>GFKQDIATLRGDLRTYAQDIFLAFLNKFPDEKRNFKNYVGKSDQELKSMAKFGDHTEKVFNLMMEVADRATDCVPLASDASTLVQMKQHSGLTTGNFEKLFVALVEYMRASGQSFDSQSWDRFGKNLVSA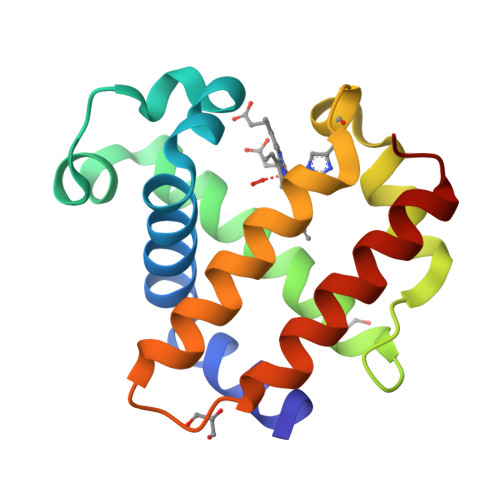LSSAGMK[2x]> MAEYQDKVVDVEVSLGTQPIDTVGFETPMFLAMHGNFPERIRFYVSTAGMVADGFAVGSPAYQFATNAFAGNFAPQRVAIGRMSIDSSKVDFTGTTNTEQVVVNITLNKVVKAVKINVLPGNTPAQIATALADAVTADADLTGKATAVATGTYVTVTAVSPNVVSVGKGAGVYKIVNESSETVATVLPSVIAENHNWYFLATEARSDADIVAAAEFAKANYKLHIYNSTDVDAYAPENSAASVFDTLKSLSYDSLGTSDAGADVDFTEGSVIGAMAANDPSYGDSLHLKTMPGMVPFAGSDTQRSNAWSRNANIYRGLYGGGSYIE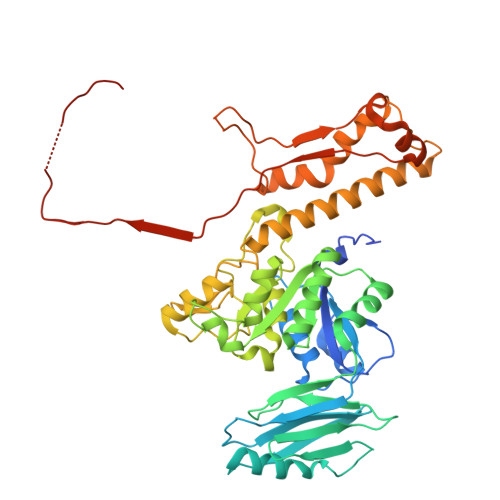GKTSSGQYVDVIRFSHWVKFRMEESVFAYMKRRSDMGLSMKMSDEDLPVLKSVLMNNPINIGIRNGGILTGYDTENKVSYDPTIIIPKRANIPTNDLAARILRDVKVELVYNNSLHYVKIRASVVLDRPAGQSTNAQTPMSSSAVGV> MDSTGASQIVSALDVIYSPKSNNSQRQEAQKFLDEVKLCSESPFWGYEIALQNPTNSILKYFGLGLLDHAVKKNWNDYDEGKRVALRKWVMELNFGVQDYDTRYIKEKLATLWVEVAKRTWGEALKQTNPTEEQLLTSWVDMDNNLFELWNINQSSRELALIIFRILFEDVFLLDDLIVLKRMTVIQPLCVMIVCPIEVFAIKYKFSDKWTKFKANEEGWFSVWIPELNNALQQNNSEYIIRLLETLKTCLNWPLTEVIVRNDVLSSLLTCLSSNIPRAQSMALDSIHILLTRPYSNESHYQMTIDRVFDNMDLLDSVYESLLFDPTDDIDETKYPIIKKFVDMISCLYVCVPKIKETNGQIQKYFKLVLKTTYNPSLIVSGLTLDLWCTCLRNDEYLPKLEKYVIPDLLQFAADALVYYEQIDGHISKKFAEIDFQSKSEFQTFCSTYRKRIRDIIRLISCVELDLTYDWLNNRLNNYFSSPFGQQVLSSTFLDHKLEPYLGALSQYMIVECFINGCIRWKIWYPTGDDYDEKLDSILQKLEILSNQLIALNLREPLLLKKQIQNFALFLTMLKDNVLFTLLEKIITSATMDYPEINLEERGAESDAVRDLRYACGIELNRMALLMPESLKKIYPDLESVIARIMPNLSYHEKISFKSFLLIIVLKSSLDMKEERFAAIVDPELLAWSDKTTVVGLSDLHWFMERLGIVQIAEYFQRRDIDENSDLLSIPIDDEGKELKSELTKRWQSLFPVRATRMFIHYSMQSIKTDEEFKMLQDLWRPRIVPILPYITRLLYQLQSYHDPDNWKGLP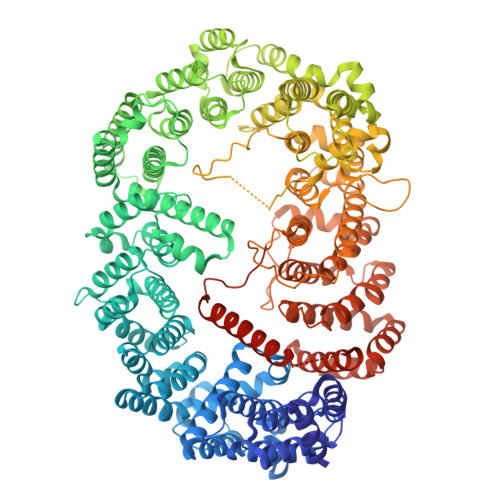TVVQSFVKYSTIERFWEAGASNKSKDEFIDEHMKAMQTLRDFADSVGHIIRYTREYTLLVLSAISSLGSVFYLLDESPDLLLNSIAIFKPGSNEISPGVSTHGWKHIMNIAIRPILKGCPKDCLGKFMPAFLPKLFEILDLLLCQKWSSHMNDMDMNPVPTDDDQMTEEILEENLLRQLTTVVVRIVIDCVGQGNANPNSAKSRLNNHQMEMRKIIFNDLNTLAPFLKLLNHLISFKDTKCSFNSILVMKCCLTSVLNQNNTVDEYFTFEVMKNLLLNVLCNSAFKDSFHEALYAFTVIFLTLCKEYPSARAFLFEISNGYNIDELYRNLRSVDEYKTQRALMIDFIDWVKSTSGKEDGNVDHAGDERKRQEKREAILKKANERLIKKNKENGDMLDDPNIEDGAVGNLFDDNENLYFQ>[12x]MEINIGIGEQDRAAIAEGLSRLLADTYTLYLKTHNFHWNVTGPMFNTLHLMFEGQYTELAVAVDDIAERIRALGFPAPGTYAAYARLS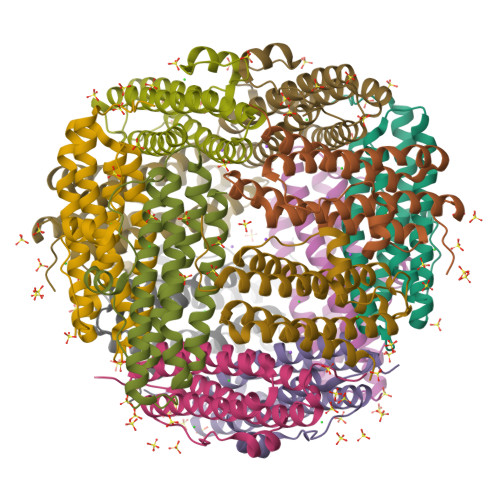SIKEEEGVPEAEEMIRQLVQGQEAVVRTARSIFPLLDKVSDEPTADLLTQRMQVHEKTAWMLRSLLAS> GPMDQYKEEDSTVSILPTSLPQIHRANMLAQGSPAASKISPLVTKKSKTRWHFGIRSRSYPLDVMGEIYIALKNLGAEWAKPSEEDLWTIKLRWKYDIGNKTNTNEKIPDLMKMVIQLFQIETNNYLVDFKFDGWESSYGDDTTVSNISEDEMSTFSAYPFLHLTTKLIMELAVNSQSN;> MEYTTDIPAVFTDPSVMERYYYTLDRQQSNTDTSWLTPPQLPPQLENVILNKYYATQDQFNENNSGALPIPNHVVLNHLVTSSIKHNTLCVASIVRYKQKYVTQILYTPIESS;> MAKPTQDSQEKVSIE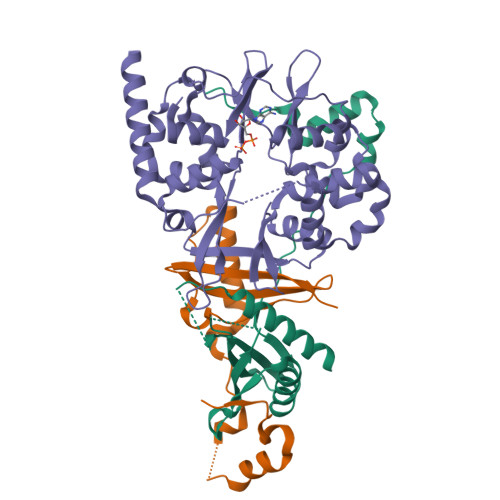QQLAVESIRKFLNSKTSYDVLPVSYRLIVLDTSLLVKKSLNVLLQNSIVSAPLWDSKTSRFAGLLTTTDFINVIQYYFSNPDKFELVDKLQLDGLKDIERALGVDQLDTASIHPSRPLFEACLKMLESRSGRIPLIDQDEETHREIVVSVLTQYRILKFVALNCRETHFLKIPIGDLNIITQDNMKSCQMTTPVIDVIQMLTQGRVSSVPIIDENGYLINVYEAYDVLGLIKGGIYNDLSLSVGEALMRRSDDFEGVYTCTKNDKLSTIMDNIRKARVHRFFVVDDVGRLVGVLTLSDILKYILLGSN> GPGSMAEMKTDAATLAQEAGNFERISGDLKTQIDQVESTAGSLQGQWRGAAGTAAQAAVVRFQEAANKQKQELDEIST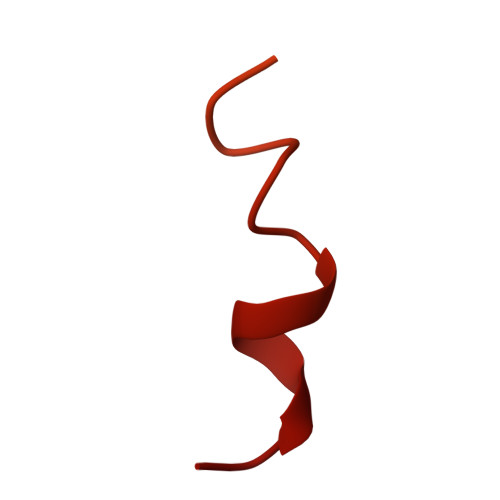NIRQAGVQYSRADEEQQQALSSQMGF>[18x]LNGRGSTTSMRGVVKLTTTAGSQSGGDASSALAWNADVIHQRGGQTINGTL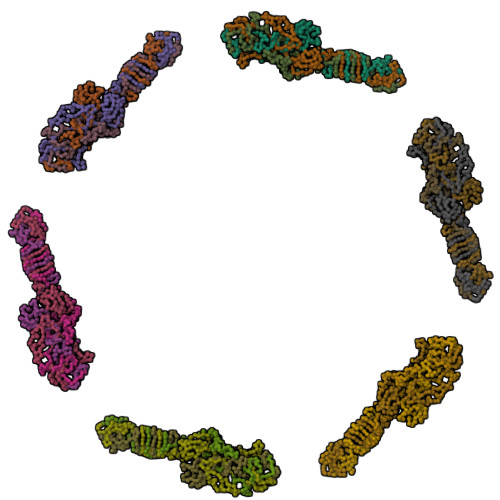RINNTLTIASGGANITGTVNMTGGYIQGKRVVTQNEIDRTIPVGAIMMWAADSLPSDAWRFCHGGTVSASDCPLYASRIGTRYGGSSSNPGLPDMRGLFVRGSGRGSHLTNPNVNGNDQFGKPRLGVGCTGGYVGEVQIQQMSYHKHAGGFGEHDDLGAFGNTRRSNFVGTRKGLDWDNRSYFTNDGYEIDPESQRNSKYTLNRPELIGNETRPWNISLNYIIKVKE> MGKDQLVIDAGQKHFGTT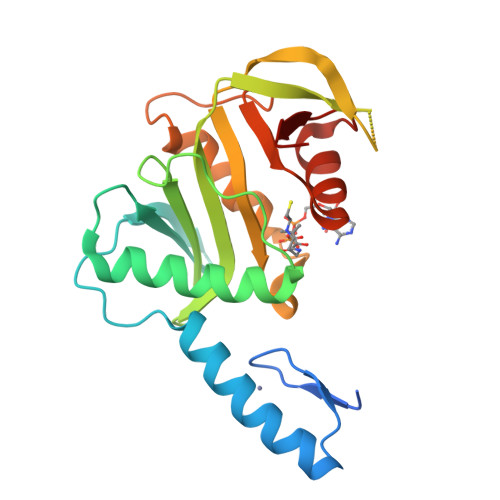VCKSCGMIYTASNPEDEIQHLQHHHRFLEGIKFVGWKRERVVAEFWDGKIVLVLPRDPSYAIKKVEDVQELVDLELGFQQTVPVCPDKTKTFLFIDEKRVVGCLIAEPIKQAFRVLSEPSASKECSRAWRCSDVPEPAICGISRIWVFRLKRRKRIARRLVDTVRNCFMFGCFLSTNEIAFSDPTPDGKLFATKYCNTPNFLVYNFHN>[4x]GPGLKQKIVIKVAMEGNNCRSKAMALVASTGGVDSVALVGDLRDKIEVVGYGIDPIKLISALRKKVGDA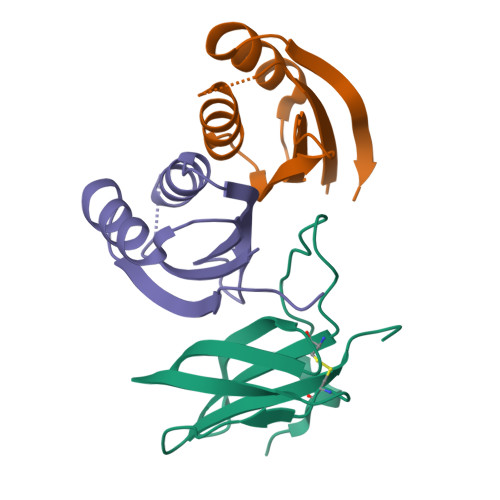ELLQVSQANKD;>METGNKYIEKRAIDLSRERDPNFFDNPGIPVPECFWFMFKNNVRQDAGTCYSSWKMDMKVGPNWVHIKSDDNCNLSGDFPPGWIVLGKKRPGF[2x]>MAHHHHHHSSGLEVLFQGPMTHSVVELIEIESAIIQVKMQDRTHKNAFSQELTDDLIQAFEYIRQNPKYKAVILTGYDNYFASGGTQEGLLRIQQGLTKFTDDNLYSLALDCEIPVIAAMQGHGIGGGFVMGLFADIVILSRESVYTANFMKYGFTPGMGATFIVPKKLGFSLAQEILLNAGSYRGADLEKRGVPFKVLP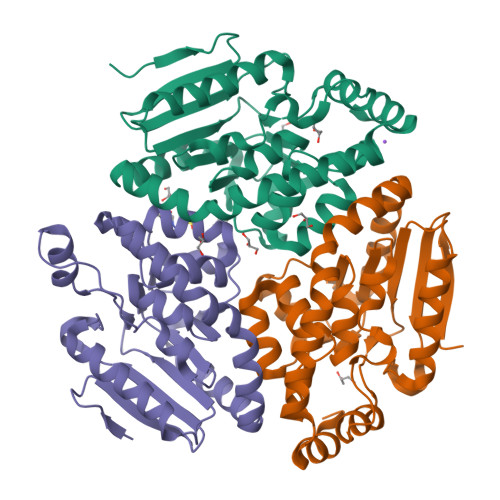RAEVLDYAVELAQELAEKPRNSLVTLKDHLVAPLRDQLPRVIEQELMMHEKTFHHEEVKSRIKGLYGN[3x]> MNTYAQESKLRLKTKIGADGRCVIEDNFFTPPFKLMAPFYPKDDLAEIMLLAVSPGMMRGDAQDVQLNIGPNCKLRITSQSFEKIHNTEDGFASRDMHIVVGENAFLDFAPFPLIPFENAHFKGNTTISLRSSSQLLYSAIIVAGRVARNELFKFNRLHTKISILQDEKPIYY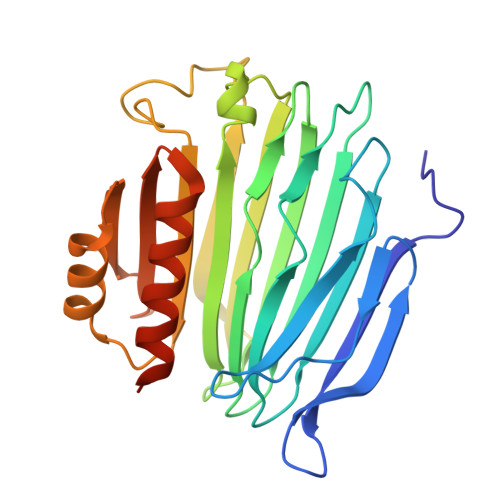DNTILDPKTTDLNNMCMFDGYTHYLNLVLVNCPIELSGVRECIEESEGVDGAVSETASSHLCVKALAKGSEPLLHLREKIARLVTQTTTQKVWSHPQFEK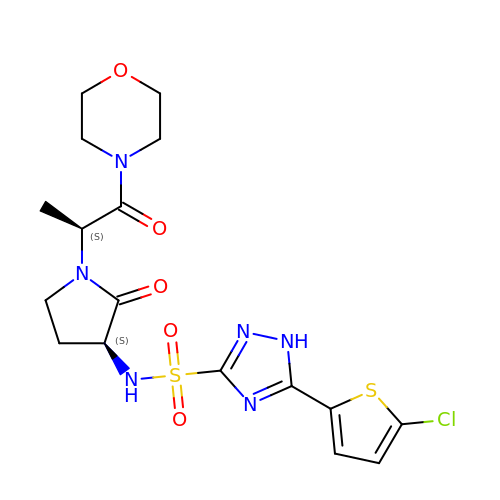5-(5-CHLORO-2-THIENYL)-N-{(3S)-1-[(1S)-1-METHYL-2-MORPHOLIN-4-YL-2-OXOETHYL]-2-OXOPYRROLIDIN-3-YL}-1H-1,2,4-TRIAZOLE-3-SULFONAMIDE | C17 H21 Cl N6 O5 S2 | FKCQUVAGEOSYRU-QWRGUYRKSA-N> MSLQMVTVGHNIALIQPGFSLMNFDGQVFFFGQKGWPKRSCPTGVFHFDIKQNHLKLKPAIFSKDSCYLPPLRYPATCSYKGSIDSDKHQYIIHGGKTPNNELSDKIYIMSVACKNNKKVTFRCTEKDLVGDVPEPRYGHSIDVVYSRGKSMGVLFGGRSYMPSTQRTTEKWNSVADCLPHVFLIDFEFGCATSYILPELQDGLSFHVSIARNDTVYILGGHSLASNIRPANLYRIRVDLPLGTPAVNCTVLPGGISVSSAILTQTNNDEFVIVGGYQLENQKRMVCSLVSLGDNTIEI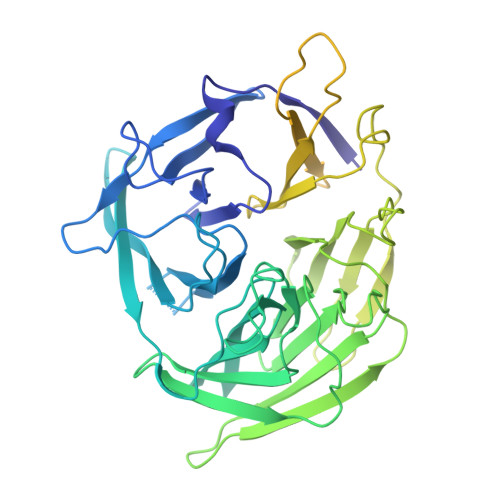SEMETPDWTSDIKHSKIWFGSNMGNGTIFLGIPGDNKQAMSEAFYFYTLRCSEEDLSEDQKIVSNSQTSTEDPGDSTPFEDSEEFCFSAEATSFDGDDEFDTYNEDDEDDESVTGYWITCCPTCDVDINTWVPFYSTELNKPAMIYCSHGDGHWVHAQCMDLEERTLIHLSEGSNKYYCNEHVQIARALQAPKRNPPLQKPPMKSLHKKGSGKVLTPAKKS(2R,4S)-2-[(1S)-1-{[(2R)-2-carboxy-2-(thiophen-3-yl)acetyl]amino}-1-methoxy-2-oxoethyl]-5,5-dimethyl-1,3-thiazolidine-4-carboxylic 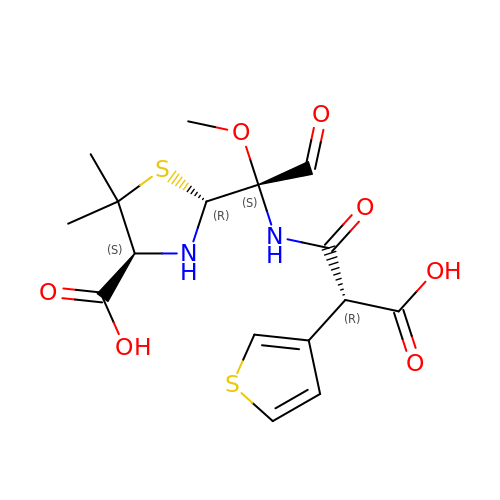acid | C16 H20 N2 O7 S2 | DGNYADVSOUQAEQ-LCFNMQHZSA-N> SNVPAELKYSKEHEWLRKEADGTYTVGITEHAQELLGDM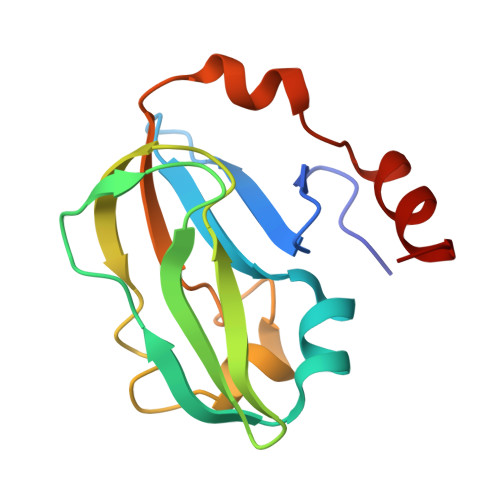VFVDLPEVGATVSAGDDCAVAESVKAASDIYAPVSGEIVAVNDALSDSPELVNSEPYAGGWIFKIKASDESELESLLDATAYEALLEDE> MSLPEILPLEVIDKTINQKVLIVLQSNREFEGTLVGFDDFVNVILEDAVEWLIDPEDESRNEKVMQHHGRMLLSGNNIAILVPG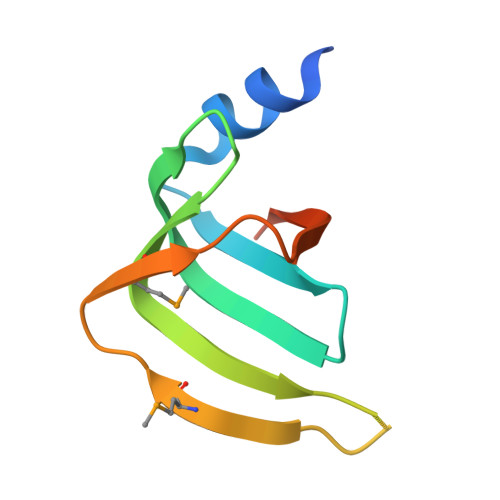GKKTPTEAL> SRKTYTLTDYLKNTYRLKLYSLRWISDHEYLYKQENNILVFNAEYGNSSVFLENSTFDEFGHSINDYSISPDGQFILLEYNYVKQWRHSYTASYDIYDLNKRQLITEERIPNNTQWVTWSPVGHKLAYVWNNDIYVKIEPNLPSYRITWTGKEDIIYNGITDWVYEEEVF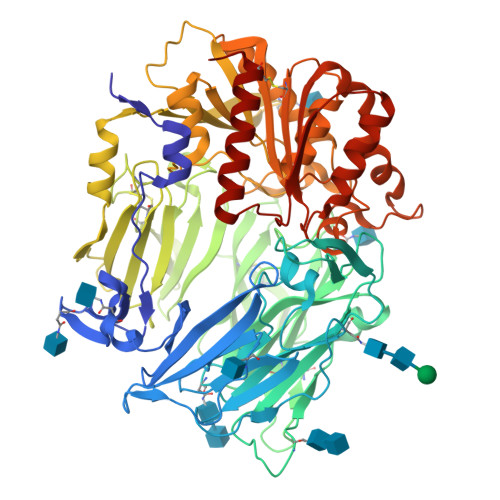SAYSALWWSPNGTFLAYAQFNDTEVPLIEYSFYSDESLQYPKTVRVPYPKAGAVNPTVKFFVVNTDSLSSVTNATSIQITAPASMLIGDHYLCDVTWATQERISLQWLRRIQNYSVMDICDYDESSGRWNCLVARQHIEMSTTGWVGRFRPSEPHFTLDGNSFYKIISNEEGYRHICYFQIDKKDCTFITKGTWEVIGIEALTSDYLYYISNEYKGMPGGRNLYKIQLSDYTKVTCLSCELNPERCQYYSVSFSKEAKYYQLRCSGPGLPLYTLHSSVNDKGLRVLEDNSALDKMLQNVQMPSKKLDFIILNETKFWYQMILPPHFDKSKKYPLLLDVYAGPCSQKADTVFRLNWATYLASTENIIVASFDGRGSGYQGDKIMHAINRRLGTFEVEDQIEAARQFSKMGFVDNKRIAIWGWSYGGYVTSMVLGSGSGVFKCGIAVAPVSRWEYYDSVYTERYMGLPTPEDNLDHYRNSTVMSRAENFKQVEYLLIHGTADDNVHFQQSAQISKALVDVGVDFQAMWYTDEDHGIASSTAHQHIYTHMSHFIKQCFSLP;> ECDFSPLLSGTPPQVYNFKRLVFTNCNYNLTKLLSLFSVNDFTCSQISPAAIASNCYSSLILDYFSYPLSMKSDLSVSSAGPISQFNYKQSFSNPTCLILATVPHNLTTITKPLKYSYINKCSRLLSDDRTEVPQLVNANQYSPCVSIVPSTVWEDGDYYRKQLSPLEGGGWLVASGSTVAMTEQLQMGFGITVQYGTDTNSVC>[4x]MPIKVGINGFGRIGRMVFQALCEDGLLGTEIDVVAVVDMNTDAEYFAYQMRYDTVHGKFKYEVTTTKSSPSVAKDDTLVVNGHRILCVKAQRNPADLPWGK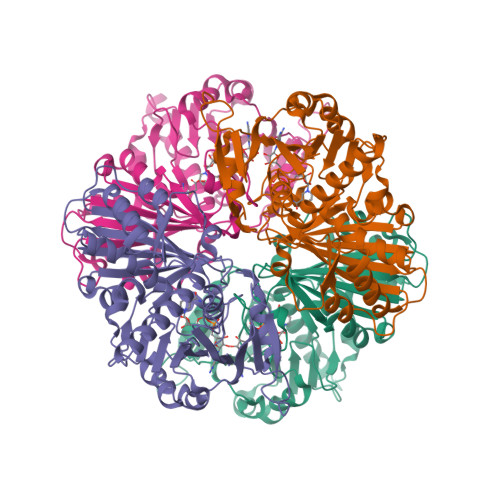LGVEYVIESTGLFTAKAAAEGHLRGGARKVVISAPASGGAKTLVMGVNHHEYNPSEHHVVSNASCTTNCLAPIVHVLVKEGFGVQTGLMTTIHSYTATQKTVDGVSVKDWRGGRAAAVNIIPSTTGAAKAVGMVIPSTQGKLTGMSFRVPTPDVSVVDLTFTAARDTSIQEIDAALKRASKTYMKGILGYTDEELVSADFINDNRSSIYDSKATLQNNLPKERRFFKIVSWYDNEWGYSHRVVDLVRHMASKDRSARL>MSLTTSKTRKSGVAMTEKLELDPARTAIVLIEYQNEFTSDGGVLHGAVADVMQHTGMLANTVAVVDAARQAGVPIMHAPITFA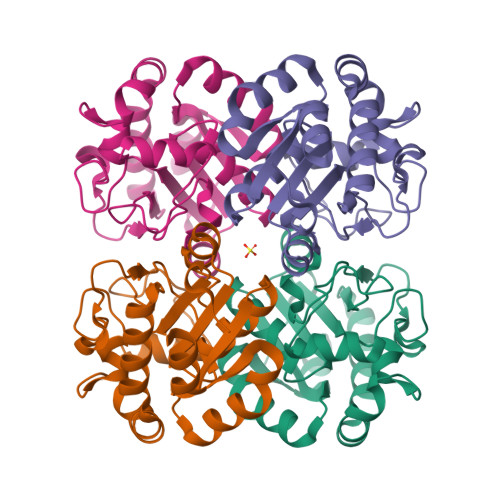EGYGELTRHPYGILKGVVDGKAFVKGTWGAAIVDELAPVNGDIVIEGKRGLDTFASTNLDFILRSKGVDTIVLGGFLTNCCVESTMRTGYERGFRVITLTDCVAATSQEEHNNAISYDFPMFSVPMTSADVIAALEGHHHHHH[12x]MALATE LIKE INTERMEDIATE | C4 H4 O5 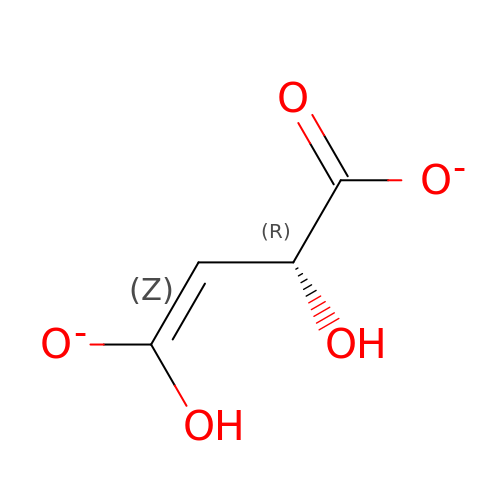| QFBHYOKSQPPXHZ-UWTATZPHSA-L> APDTSVSNKQNFSTDVIYQIFNDRFSDGNPANNPTGAAFDGTCTNLRLYCGGDWQGIINKINDGYLTGMGVTAIWISQPVENIYSIINYSGVNNTAYHGYWARDFKKTNPAYGTIADFQNLIAAAHAKNIKVIIDFAPNHTSPASSDQPSFAENGRLYDNGTLLGGYTNDTQNLFHHNGGTDFSSYEDGIYRNLYDLADLNHNNSTVDVYLKDAIKMWLDLGIDGIRMDAVKHMPFGWQKSFMAAVNNYKPVFTFGEWFLGVNEVSPENHKFANESGMSLLDFRFAQKVRQVFRDNTDNMYGLKAMLEGSAADYAQVDDQVTFIDNHDMERFHASNANRRKLEQALAFTLTSRGVPAIYYGTEQYMSGGTDPDNRARIPSFSTSTTAYQVIQKLAPLRKSNPAIAYGSTQERWINNDVLIYERKFGSNVAVVAVNRNLNAPASISGLVTSLPQGSYNDVLGGLLNGNTLSVGSGGAASNFTLAAGGTAVWQYTAATATPTIGHVGPMMAKPGVTITIDGRGFGSSKGTVYFGTTAVSGADITSWEDTQIKVKIPAVAGGNYNIKVANAAGTASNVYDNFEVLSGDQVSVRFVVNNATTALGQNVYLTGSVSELGNWDPAKAIGPMYNQVVYQYPNWYYDVSVPAGKTIEFKFLKKQGSTVTWE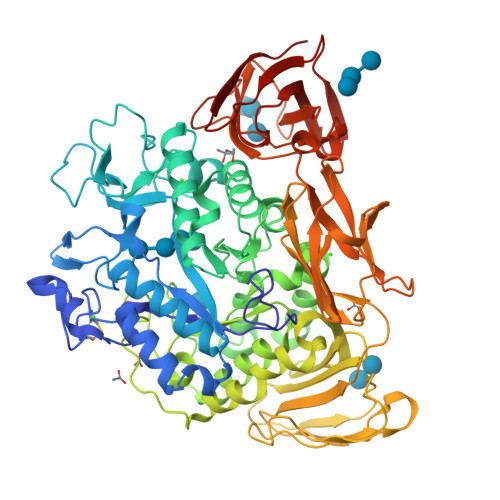GGSNHTFTAPSSGTATINVNWQP>[2x]ENPYERGPDPTESSIEAVRGPFAVAQTTVSRLQADGFGGGTIYYPTDTSQGTFGAVAISPGFTAGQESIAWLGPRIASQGFVVITIDTITRLDQPDSRGRQLQAALDHLRTNSVVRNRIDPNRMAVMGHSMGGGGALSAAANNTSLEAAIPLQGWHTRKNWSSVRTPTLVVGAQLDTIAPVSSHSEAFYNSLPSDLDKAYMELRGASHFVSNTPDTTTAKYSIAWLKRFVDNDLRYE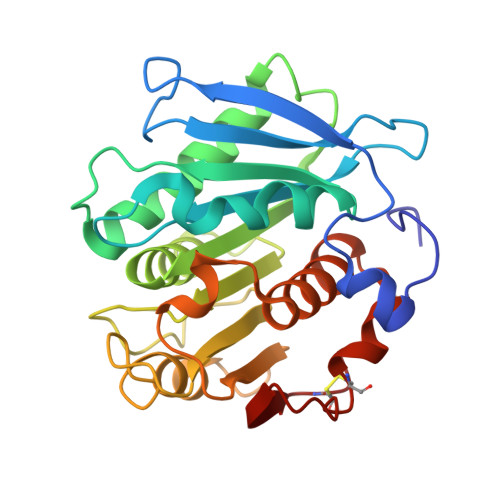QFLCPAPDDFAISEYRATCPF(3-{[(3-chloro-2-hydroxyphenyl)sulfonyl]amino}phenyl)acetic 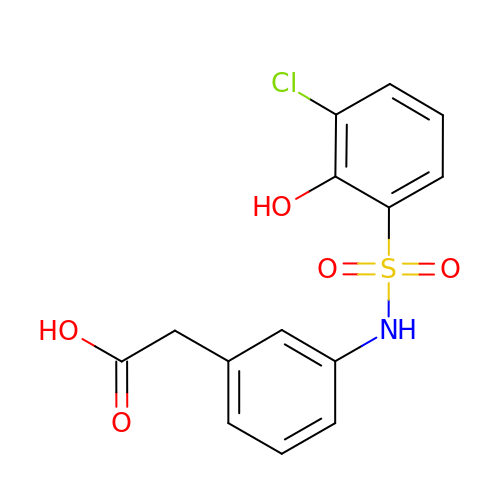acid | C14 H12 Cl N O5 S | KIHNFFHPSDCHNU-UHFFFAOYSA-N>[3x]MKKIEAIVRAEKFPEVKAALEERGFYGMTVTDVKGRGQQGGMQI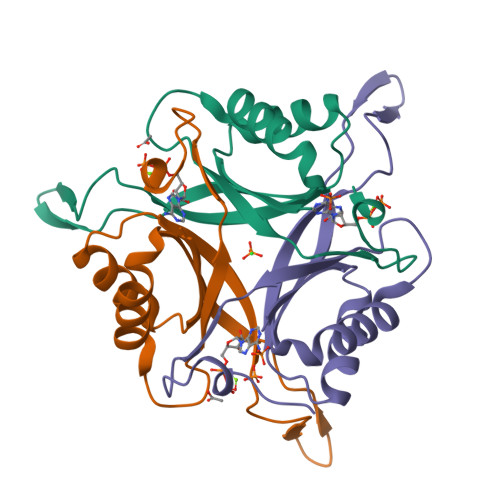QFRGRTMEVTLLPKVKLEIVVKDDAVEEVIGLIVNSAFTGSPGDGKIFIIPVEDVVRIRTGERGDDSLEHHHHHH> 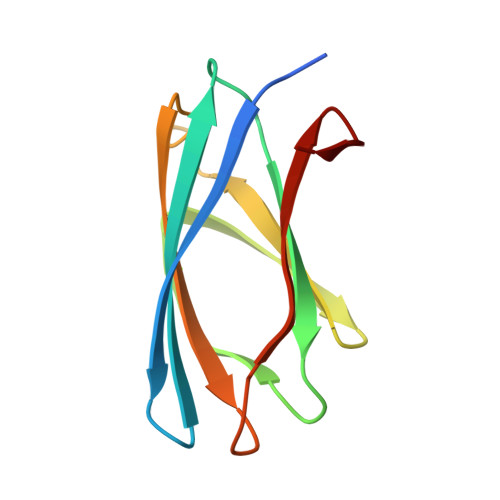GPTTPVPVSGSLEVKVNDWGSGAEYDVTLNLDGQYDWTVKVKLAPGATVGSFWSANKQEGNGYVIFTPVSWNKGPTATFGFIVNGPQGDKVEEITLEINGQVI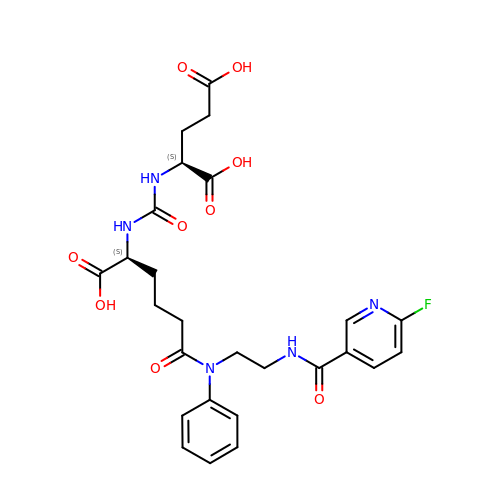(2~{S})-2-[[(2~{S})-6-[2-[(6-fluoranylpyridin-3-yl)carbonylamino]ethyl-phenyl-amino]-1-oxidanyl-1,6-bis(oxidanylidene)hexan-2-yl]carbamoylamino]pentanedioic acid | C26 H30 F N5 O9 | AFDHXMJDHQVEHD-OALUTQOASA-N>GSMGAEIPKEMLRAQTNVILLNVLKQGDNYVYGIIKQVKEASNGEMELNEATLYTIFDRLEQDGIISSYWGDESQGGRRKYYRLTEIGHENCRLAFESWSRVRKI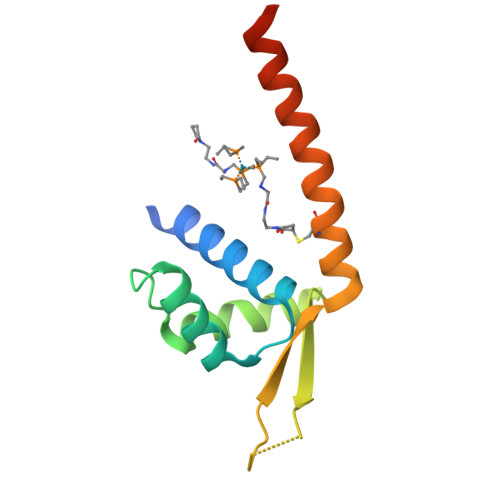IENLEANKKSEAIK[2x]> MISNFRKFHGNKNQEKFNENLILNKENESILNYLDPICKTLEIIPEITYLGSSVEPINKVYKFNKEEKTSDIERSELQLIKMSFLIEKDDKKEEINKFIYFPKLIDSQYFIINGNRYYPIYQLLDSGTYRTNKALTLKTLLMPIVLREKKETFDDINGETHTMLNVDLDLFKSKVPFLIYFFSKFGFEGTLEYFGLQDLIHVLMKEDLDQLDEDEINDNV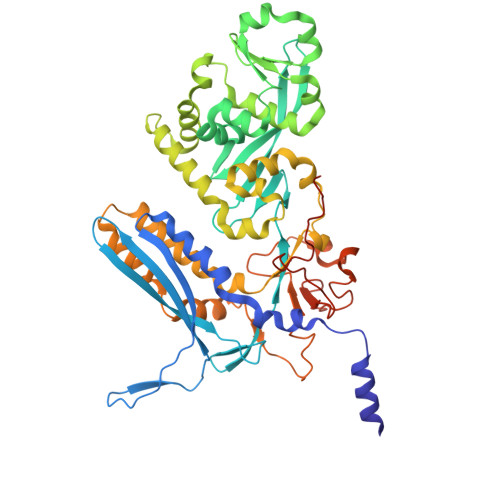IFMITKNISLVVDKNFFSNKNNQIIIATLLNCFNTRIKIDKIYEKDYWVKKLGGYFTTNNSNKQEKGEGIILSFERILDEWTKKILRTEEKNKEDIYSVVRWMINNYLALVKQDNMNLANKRIRLYEYLLHPLLIKFSKGTYRVLNNRNSNKFEKIKTIFSNIQEGFLVKKIINNELLRYDNSVNSISLFTLILRYTQSGPQSPFSSNSTNNKLRGLHPSYLGRLGLTSTSAGDPGASGSLTPFLELPENSYMHFTEEPEINLNIDDISIDEVIES> GKHTVPYTISVDGITALHRTYFVFPENKKVLYQEIDSKVKNELASQRGVTTEKINNAQTATYTLTLNDGNKKVVN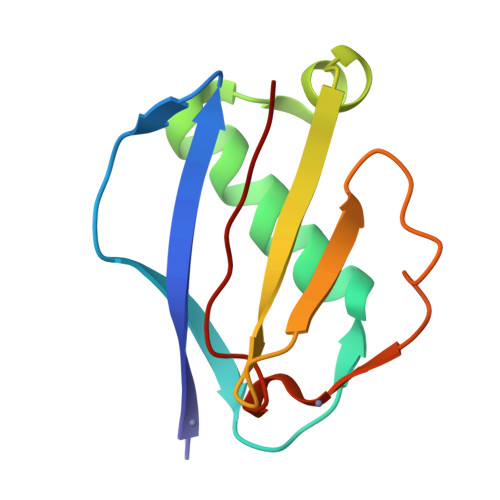LKKNDDAKNSIDPSTIKQIQIVVK S-layer proteins (SLPs) are self-assembling, crystalline proteins coating the cell surfaces of many prokaryotes. We determined the atomic resolution structures of all functional domains (I-III from N- to C-termini) present in the three S-layer proteins SlpA_ac, SlpX_ac, and SlpA_amy. The Lactobacillus S-layers are anchored to the cell wall through interaction with teichoic acids (TA), either lipoteichoic acid (LTA) or wall teichoic acid (WTA).

The full-length SlpX_ac shows differences in structure and domain arrangement compared to the SlpA architecture. The middle domain of SlpX, SlpX_ac_II, exhibits a SlpA_I-like domain fold and an additional repeat of the SlpA motif. The four residues observed in the vicinity of phosphates are conserved with the proposed binding motif of YxY….KxxN. These residues are not conserved in the third SlpA-motif, which is present in SlpX_ac_II. However, SlpX_ac_II contains an additional 3rd SlpA motif and an additional loop region, allowing for increased protein flexibility to incorporate into the assembled SlpA-SlpX S-layer. In summary, the atomic structures of Lactobacillus S-layer proteins, SlpA and SlpX, along with the observed differences in their domain organization, enabled us to generate a self-assembly model for SlpA, the main SLP. This model aligns with prior studies and suggests a domain-swapping mechanism that enables the integration of SlpX into the S-layer.

>MGSTPTDTTQNPQINWTKGGQAQSSSLNGQVFQVAVGSNFNPLNFTNSNGENIIVSAQQSKNNTTFASIEATSNPVNTSEAGRYYNVTLTATGNTGKKTTATYTVLITSSQKQTLYGNGESTISTYSIYGNNVLSNSTTFKDGDQVYVSDQTKTVGGVSYSQVSPKSKNDANSSNIWVKTSLEHHHHHH[6x]> MIKVEIKPSQAQFTTRSGVSRQ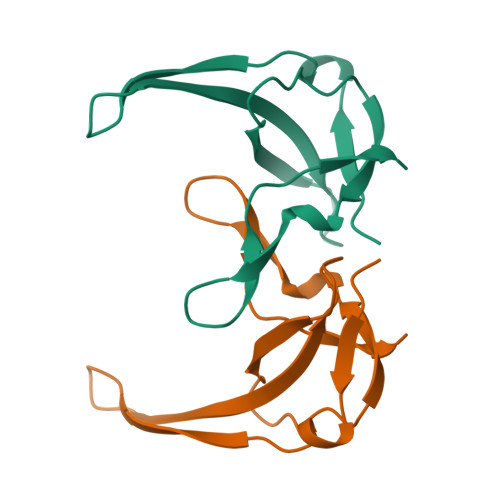GKPYSLNEQRCYVDLGNEYPVLVKITLDEGQPAYAPGLYTVHLSSFKVGQFGSLMIDRLRLVPAK> YLGSRDHFALDRPSETHADYLLRTGQVVDISDTIYPRNPAMYSEEARLKSFQNWPDYAHLTPRELASAGLYYTGIGDQVQCFCCGGKLKNWEPCDRAWSEHRRHFPNCFFVLGRNLNIRSESD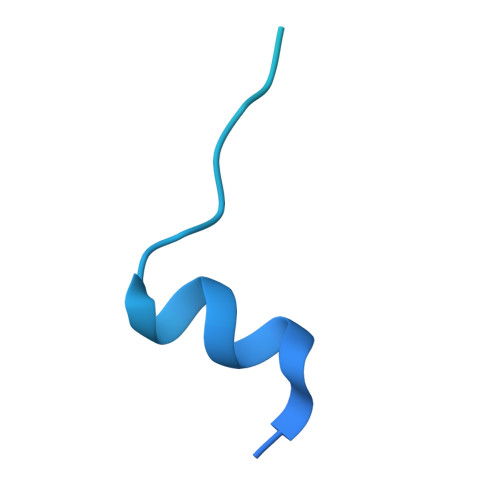AVSSDRNFPNSTNLPRNP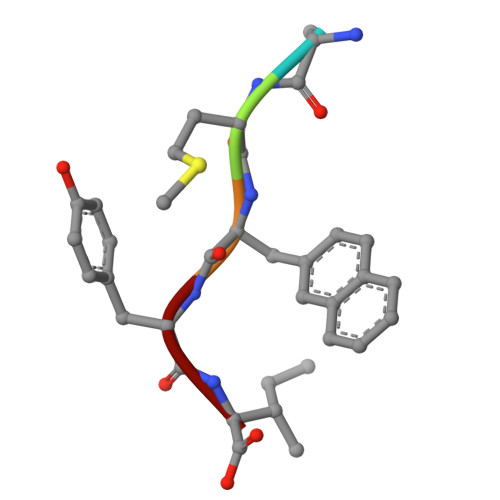> YMAYI> XSGRGKGGKGL;> GPLGSPEFMAQGTLIRVTPEQPTHAVCVLGTLTQLDICSSAPEDCTSFSINASPGVVVDIAHSPPAKKKSTGSSTWPLDPGVEVTLTMKAASGSTGDQKVQISYYGPKTPPVKALLYLTAVEISLCADITRTGKVKPTRAVKDQRTWTWGPCGQGAILLVNCDRDNLESSAMDCEDDEVLDSEDLQDMSLMTLSTKTPKDFFTNHTLVLHVARSEMDKVRVFQATRGKLSSKCSVVLGPKWPSHYLMVPGGKHNMDFYVEALAFPDTDFPGLITLTISLLDTSNLELPEAVVFQDSVVFRVAPWIMTPNTQPPQEVYACSIFENEDFLKSVTTLAMKAKCKLTICPEEENMDDQWMQDEMEIGYIQAPHKTLPVVFDSPRNRGLKEFPIKRVMGPDFGYVTRGPQTGGISGLDSFGNLEVSPPVTVRGKEYPLGRILFGDSCYPSNDSRQMHQALQDFLSAQQVQAPVKLYSDWLSVGHVDEFLSFVPAPDRKGFRLLLASPRSCYKLFQEQQNEGHGEALLFEGIKKKKQQKIKNILSNKTLREHNSFVERCIDWNRELLKRELGLAESDIIDIPQLFKLKEFSKAEAFFPNMVNMLVLGKHLGIPKPFGPVINGRCCLEEKVCSLLEPLGLQCT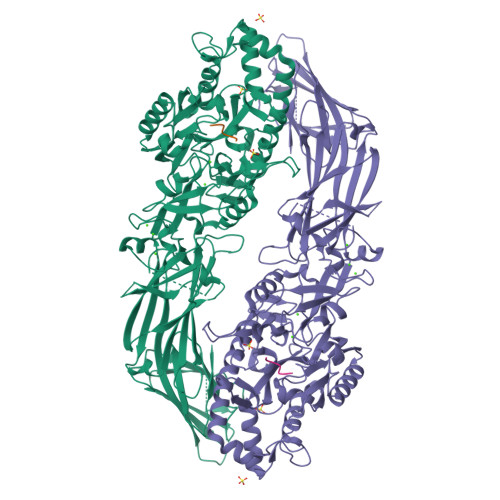FINDFFTYHIRHGEVHAGTNVRRKPFSFKWWNMVP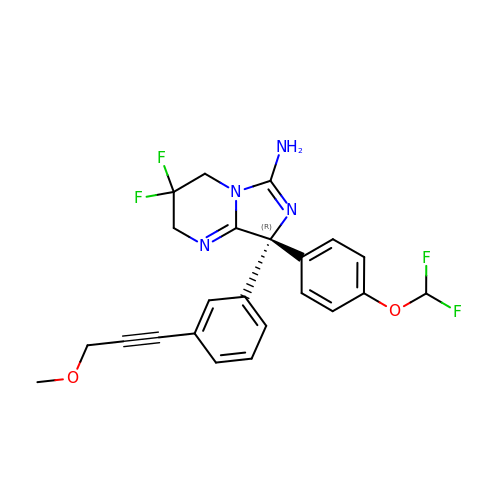(8R)-8-[4-(DIFLUOROMETHOXY)PHENYL]-3,3-DIFLUORO-8-[3-(3-METHOXYPROP-1-YN-1-YL)PHENYL]-2,3,4,8-TETRAHYDROIMIDAZO[1,5-A]PYRIMIDIN-6-AMINE | C23 H20 F4 N4 O2 | DOQWIXXNZSOWDD-HSZRJFAPSA-N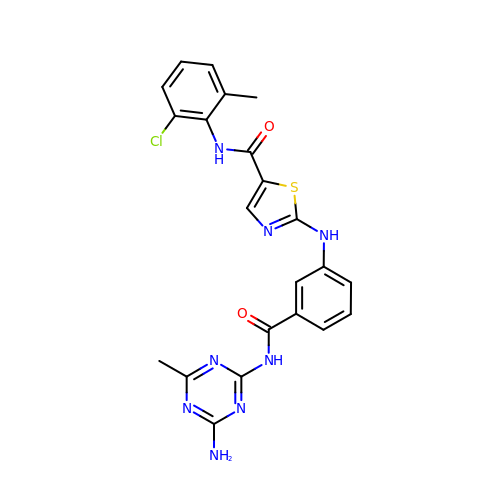2-[[3-[(4-azanyl-6-methyl-1,3,5-triazin-2-yl)carbamoyl]phenyl]amino]-~{N}-(2-chloranyl-6-methyl-phenyl)-1,3-thiazole-5-carboxamide | C22 H19 Cl N8 O2 S | BVMIJKUOTIIKFU-UHFFFAOYSA-N> AGEAWPTHTACRNGNLQVLYQSCDPLQDFGFS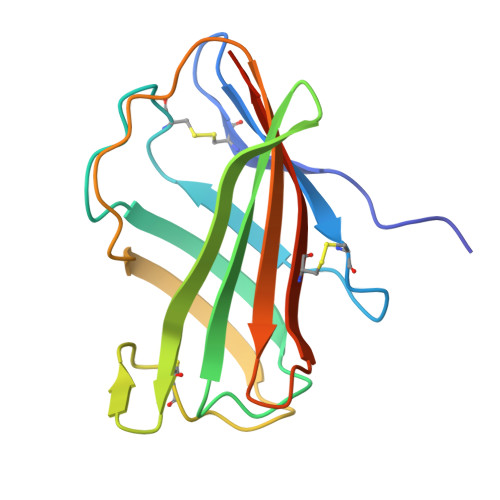VDQCARQLKPNINIRFGMVLREDIEQLFLDVALFSKGLSILNFSYPVCEVDLPKFSFCGRRKGEQIYYAGPINNPGFEIPEGDYQVLLELYNQDHATVACANATVLYSARGLVPR>[4x]STPSIVIASAARTAVGSFNGAFANTPAHELGATVISAVLERAGVAAGEVNEVILGQVLPAGEGANPARQAAMKAGVPQEATAW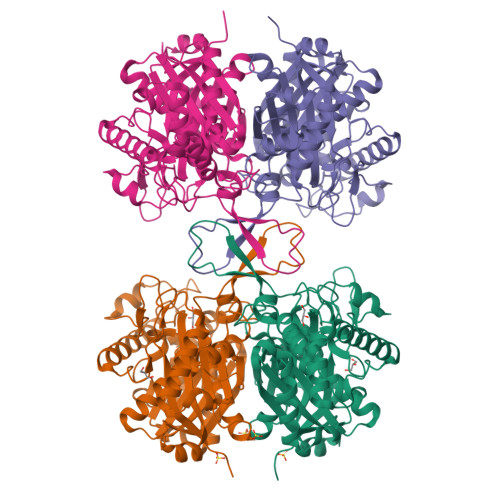GMNQLCGSGLRAVALGMQQIATGDASIIVAGGMESMSMAPHCAHLRGGVKMGDFKMIDTMIKDGLTDAFYGYHMGTTAENVAKQWQLSRDEQDAFAVASQNKAEAAQKDGRFKDEIVPFIVKGRKGDITVDADEYIRHGATLDSMAKLRPAFDKEGTVTAGNASGLNDGAAAALLMSEAEASRRGIQPLGRIVSWATVGVDPKVMGTGPIPASRKALERAGWKIGDLDLVEANEAFAAQACAVNKDLGWDPSIVNVNGGAIAIGHPIGASGARILNTLLFEMKRRGARKGLATLCIGGGMGVAMCIESL[1-[2-[3-[[(2~{R})-4-[[[(2~{R},3~{S},4~{R},5~{R})-5-(6-aminopurin-9-yl)-4-oxidanyl-3-phosphonooxy-oxolan-2-yl]methoxy-oxidanyl-phosphoryl]oxy-oxidanyl-phosphoryl]oxy-3,3-dimethyl-2-oxidanyl-butanoyl]amino]propanoylamino]ethoxy]-1-oxidanylidene-propan-2-ylidene]-bis(oxidanidyl)azanium | C24 H38 N8 O20 P3 | 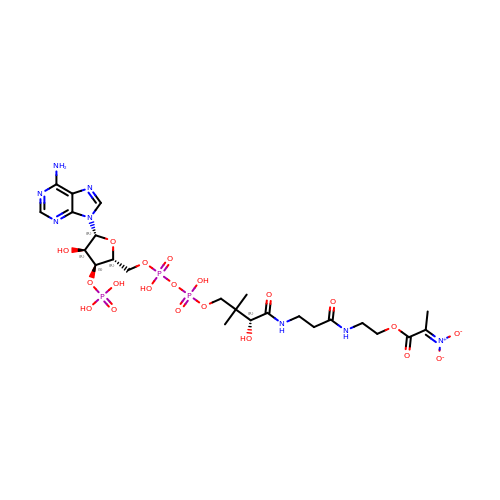JOSUZLPXQGIVES-ZSJPKINUSA-N>MAFKLPNLPYAYDALEPYIDQRTMEFHHDKHHNTYVTKLNATVEGTELEHQSLADMIANLDKVPEAMRMSVRNNGGGHFNHSLFWEILSPNSEEKGGVIDDIKAQWGTLDEFKNEFANKATTLFGSGWTWLVVNDGKLEIVTTPNQDNPLTEGKTPILLFDVWEHAYYLKYQNKRPDYMTAFWNIVNWKKVDELYQAAK[2x]

For example, Staphylococcus aureus has a constitutive Mn-specific superoxide dismutase (herein MnSOD), which is catalytically inactive when loaded with Fe, and a second one (herein camSOD)1 that is stress-induced and cambialistic—that is it can use either Mn or Fe. This cofactor promiscuity enhances the pathogenicity of S. aureus by enabling it to survive the oxidative burst of the innate immune system while experiencing host-imposed Mn starvation. Each monomer presented the characteristic fold conserved amongst Mn/Fe-SODs, with an α-helical N-terminal domain and a C-terminal α/β domain connected by a loop. The active sites were enclosed between the two domains of each monomer, with both domains contributing ligands. As shown in Fig. 3 and as expected, the Mn ions were coordinated in a distorted trigonal bipyramidal geometry by H81, D167, and H171 in the equatorial plane, and H26 and a water molecule in the axial plane.

Preparations of S. aureus MnSOD and camSOD, shown to contain exclusively Mn by ICP-MS, were used in crystallization trials. The crystal structures of Mn(Mn)SOD and Mn(cam)SOD were determined by molecular replacement, using B. subtilis SodA as a search model, at 2.07 Å and 2.30 Å, respectively (data collection and refinement statistics are provided in Table S1, ESI†). Two molecules were found in the asymmetric unit of both protein crystals. The dimers of MnSOD and camSOD were superimposable in the protein backbone with an average root mean square deviation (RMSD) of 0.744 Å by least squares fit. Most of the differences between the structures were found in the loops connecting helical elements within the N-terminal domains. S. aureus Mn(Mn)SOD and Mn(cam)SOD can be readily distinguished by their 94 GHz field-swept echo EPR spectra. For Mn(Mn)SOD, D = –10.60 and E = 0.63 GHz, similar to E. coli Mn(Mn)SOD; for Mn(cam)SOD, D = –10.66 and E = 0.43 GHz, comparable to the R. capsulatus camSOD; and for Mn(Fe)SOD, D = –10.46 and E = 0.33 GHz, which were the same within errors as those previously obtained from simulations of the Ms = –1/2 ↔ +1/2 transition. In the S. aureus Mn(Mn)SOD, the ring plane of H26 relative to the Mn–Oδ1,Asp167 bond was 180°, while in Mn(cam)SOD it was 167°. The 94 GHz ELDOR-NMR and ENDOR of Mn(Mn)SOD and Mn(cam)SOD are remarkably similar, indicating a high-degree of structural homology even at the level of the positions of the protons in proximity to the metal ion, in particular those of the water ligand.> AYAQWVIIIIHNVGSKDVKIKNLKPSWGKLHADGDKDTEVSASKYEGTVIKPDEKLQINACGRS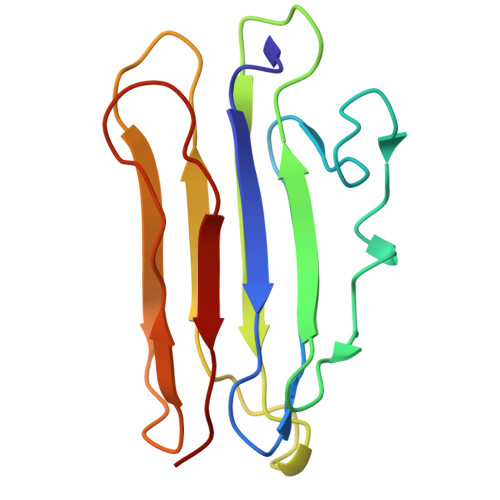DAAEGTTGTFDLVDPADGDKQVRHFYWDCPWGSKTNTWTVSGSNTKWMIEYSGQNLDSGALGTITVDTLKK>[2x]MAEGKLNDELAKNKGKIPGLKIDQKIRGQMPERGWTEDD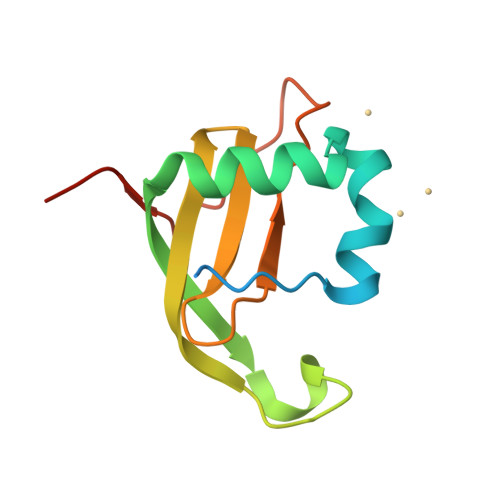IKNTVSNGATGTSFDKRSPKKTPPDYLGRNDPATVYGSPGKYVVVNDRTGEVTQISDKTDPGWVDDSRIQWGNKNDQ> MTLRAAVFDLDGVLALPAVFGVLGRTEEALALPRGLLNDAFQKGGPEGATTRLMKGEITLSQWIPLMEENCRKCSETAKVCLPKNFSIKEIFDKAISARKINRPMLQAALMLRKKGFTTAILTNTWLDDRAERDGLAQLMCELKMHFDFLIESCQVGMVKPEPQIYKFLLDTLKASPSEVVFLDDIGANLKPARDLGMVTILVQDTDTALKELEKVTGIQLLNTPAPLPTSCNPSDMSHGYVTVKPRVRLHFVELGSGPAVCLCHGFPESWYSWRYQI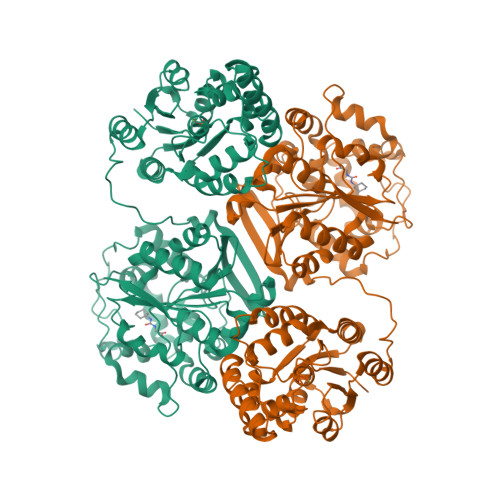PALAQAGYRVLAMDMKGYGESSAPPEIEEYCMEVLCKEMVTFLDKLGLSQAVFIGHDWGGMLVWYMALFYPERVRAVASLNTPFIPANPNMSPLESIKANPVFDYQLYFQEPGVAEAELEQNLSRTFKSLFRASDESVLSMHKVCEAGGLFVNSPEEPSLSRMVTEEEIQFYVQQFKKSGFRGPLNWYRNMERNWKWACKSLGRKILIPALMVTAEKDFVLVPQMSQHMEDWIPHLKRGHIEDCGHWTQMDKPTEVNQILIKWLDSDARNPPVVSKM>QGSIRSAEALALSDCRLHICLYYRDILVKELTTTSPEGCRISHGHTYDVSNLDQVLFPYPDDNGQRKNIEKLLSHLERGLVLWMAPDGLYAKRLCQSRIYWDGPLALCSDRPNKLERDQTCKLFDTQQFLS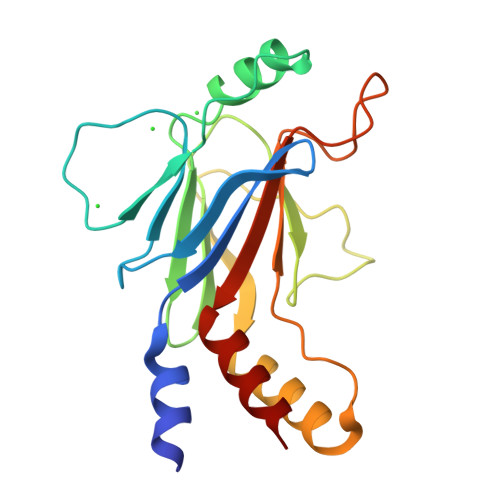ELQVFAHHGRPAPRFQVTLCFGEEFPDPQRQRKLITAHVEPLLARQLYYFAQQN[2x]>[2x]MDYKDDDDKGGSASQPPPPGPLGDCLRDWEDLQQDFQNIQETHRLYRLKLEELTKLQNNCTSSITRQKKRLQELALALKKCKPSLPAEAEGAAQELENQMKER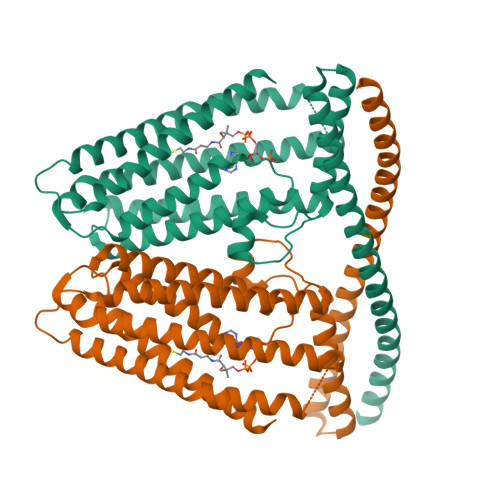QGLFFDMEAYLPKKNGLYLSLVLGNVNVTLLSKQAKFAYKDEYEKFKLYLTIILILISFTCRFLLNSRVTDAAFNFLLVWYYCTLTIRESILINNGSRIKGWWVFHHYVSTFLSGVMLTWPDGLMYQKFRNQFLSFSMYQSFVQFLQYYYQSGCLYRLRALGERHTMDLTVEGFQSWMWRGLTFLLPFLFFGHFWQLFNALTLFNLAQDPQCKEWQVLMCGFPFLLLFLGNFFTTLRVVHHKFHSQRHGSKKD>[2x]MEQNKCALVTGSSRGVGKAAAIRLAENGYNIVI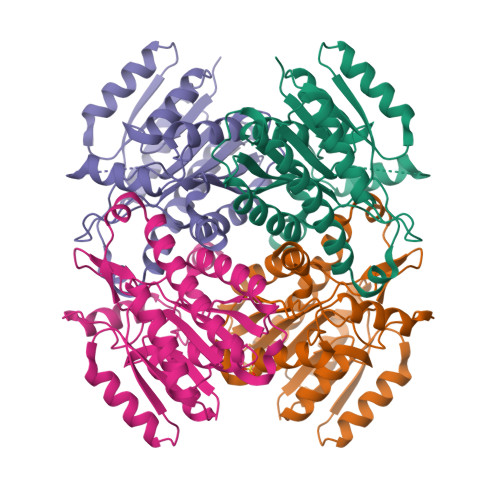NYARSKKAALETAEEIEKLGVKVLVVKANVGQPAKIKEMFQQIDETFGRLDVFVNNAASGVLRPVMELEETHWDWTMNINAKALLFCAQEAAKLMEKNGGGHIVSISSLGSIRYLENYTTVGVSKAALEALTRYLAVELSPKQIIVNAVSGGAIDTDALKHFPNREDLLEDARQNTPAGRMVEIKDMVDTVEFLVSSKADMIRGQTIIVDGGRSLLVLEHHHHHH> GSRADFFTYETPKVIVVKSWTIGIINRVVQLLIISYFVGWVFLHEKAYQVRDTAIESSVVTKVKGSGLYANRVMDVSDYVTPPQGTSVFVIITKMIVTENQMQGFCPESEEKYRCVSDSQCGPERLPGGGILTGRCVNYSSVLRTCEIQGWCPTEVDTVETPIMMEAENFTIFIKNSIRFPLFNFEKGNLLPNLTARDMKTCRFHPDKDPFCPILRVGDVVKFAGQDFAKLARTGGVLGIKIGWVCDLDKAWDQCIPKYSFTRLDSVSEKSSVSPGYNFRFAKYYKMENGSEYRTLLKAFGIRFD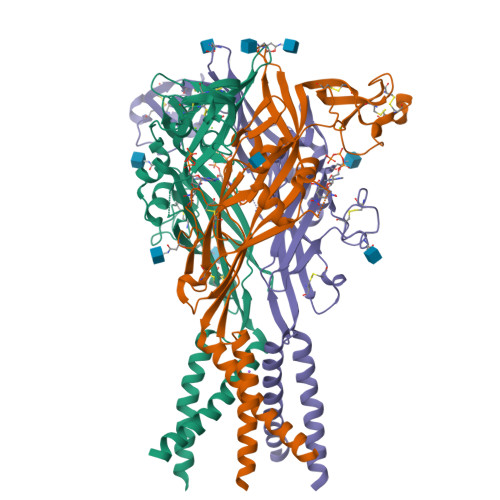VLVYGNAGKFNIIPTIISSVAAFTSVGVGTVLCDIILLNFLKGADQYKAKKFEEVNET>[2x]MSLITHFRQAIEETLPWLSSFGADPAGGMTRLLYSPEWLETQQQFKKRMAASGLETRFDEVGNLYGRLNGTEYPQEVVLSGSHIDTVVNGGNLDGQFGALAAWLAIDWLKTQYGAPLRTVEVVAMAEEEGSRFPYVFWGSKNIFGLANPDDVRNICDAKGNSFVDAMKACGFTLPNAPLTPRQDIKAFVELHIEQGCVLESNGQSIGVVNAIVGQR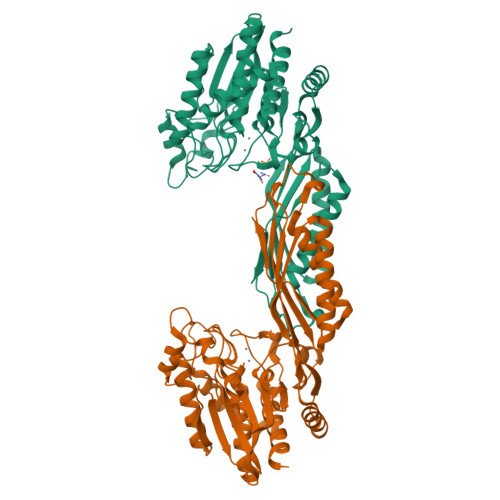RYTVTLNGESNHAGTTPMGYRRDTVYAFSRICHQSVEKAKRMGDPLVLTFGKVEPRPNTVNVVPGKTTFTIDCRHTDAAVLRDFTQQLENDMRAICDEMDIGIDIDLWMDEEPVPMNKELVATLTELCEREKLNYRVMHSGAGHDAQIFAPRVPTCMIFIPSINGISHNPAERTNITDLAEGVKTLALMLYQLAWQKEGGSHHHHHH>[4x]SYDTVRDKYWLSQYVIARETYDWYTLQKD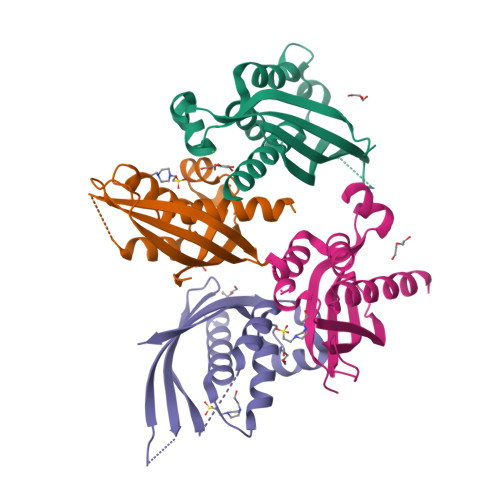YETVGMLSSPSEGQSYASQFQGDKALDKQYGSNVRTSVTIVSIVPNGKGIGTVRFAKTTKRTNETGDGETTHWIATIGYQYVNPSLMSESARLTNPLGFNVTSYRVDPEMGVV> GMLFSIQTCPCQINPALNAVSTPLLYQDCCQPYHDGLYNQEVEDSDAIRADTAEHLMRTRYSAFVLVKPEYIVKTTLPAQQDLLDIKAIENWAKE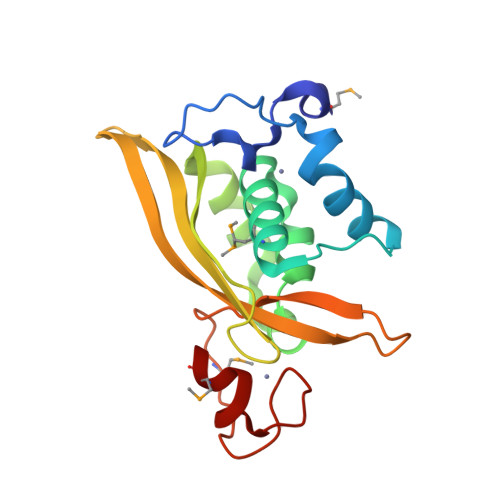TDWAGLEVVAHTPKLSKRHAQVEFKAYFKTPDGLQAHHELSTFVKIKNKANSDASWYFLDPTVSMSVTQKQPCICGSGEKFKRCCGMYI>MKVGIVGSGMVGSATAYALALLGVAREVVLVDLDRKLAQAHAEDILHATPFAHPVWVRAGSYGDLEGARAVVLAAGVAQRPGETRLQLLDRNAQVFAQVVPRVLEAAPEAVLLVATNPVDVMTQVAYRLSGLPPGRVVGSGTILDTARFRALLAEYLRVAPQSVHAYVLGEHGDSEVLVWSSAQVGGVPLLEFAEARGAALSPED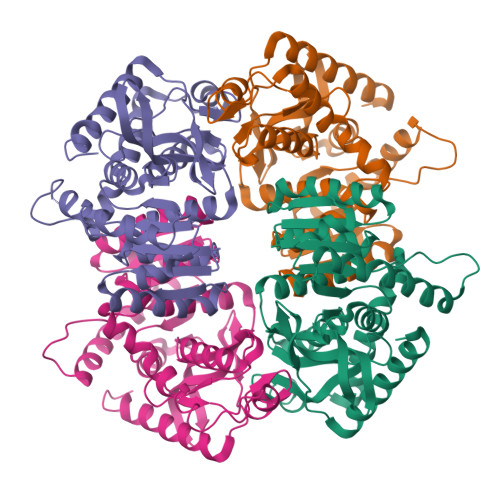RARIDEGVRRAAYRIIEGKGATYYGIGAGLARLVRAILTDEKGVYTVSAFTPEVEGVLEVSLSLPRILGAGGVEGTVYPSLSPEEREALRRSAEILKEAAFALGF[4x]~{N}-(3-cyanophenyl)-4-methyl-3-[(1-methyl-6-pyridin-3-yl-pyrazolo[3,4-d]pyrimidin-4-yl)amino]benzamide 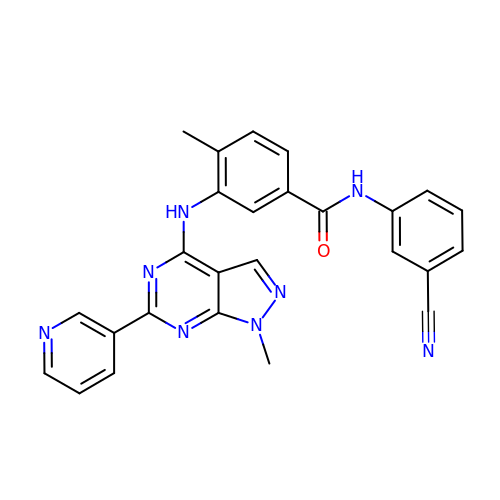| C26 H20 N8 O | ASMWZAVRNQGHAB-UHFFFAOYSA-N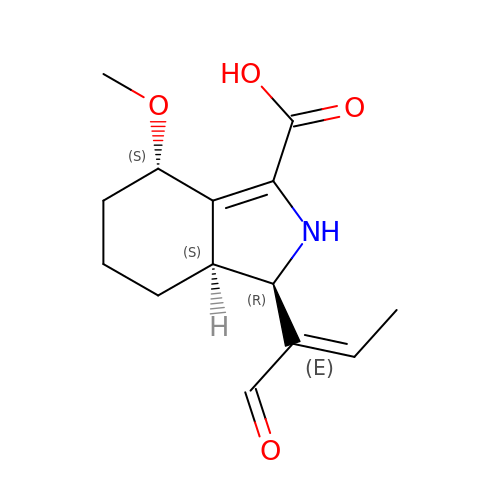(1R,4S,7AS)-1-(1-FORMYLPROP-1-EN-1-YL)-4-METHOXY-2,4,5,6,7,7A-HEXAHYDRO-1H-ISOINDOLE-3-CARBOXYLIC ACID | C14 H19 N O4 | ZYKSDPVHVMSKIL-IIHMJNQGSA-N> GANYSIVDFLI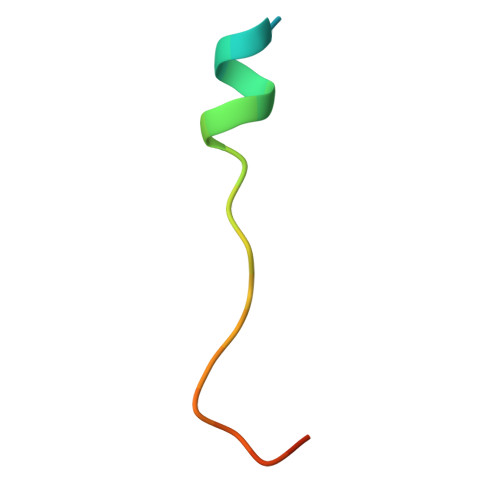TAGANVNSPDSHG> IVPDAGVGTVPMTDYGNDIEYYGQVTIGTPGKKFNLDF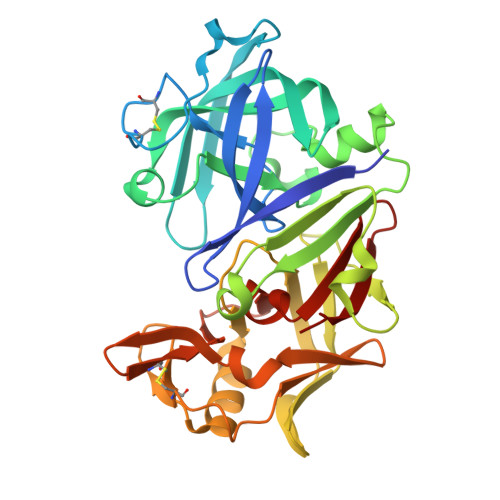DTGSSDLWIASTLCTNCGSRQTKYDPNQSSTYQADGRTWSISYGDGSSASGILAKDNVNLGGLLIKGQTIELAKREAASFANGPNDGLLGLGFDTITTVRGVKTPMDNLISQGLISRPIFGVYLGKASNGGGGEYIFGGYDSTKFKGSLTTVPIDNSRGWWGITVDRATVGTSTVASSFDGILDTGTTLLILPNNVAASVARAYGASDNGDGTYTISCDTSRFKPLVFSINGASFQVSPDSLVFEEYQGQCIAGFGYGNFDFAIIGDTFLKNNYVVFNQGVPEVQIAPVAE>GPLGSHMSTESNDGVSETLLAWRHIDFWTSEHNPDLNATLSDPCTQNDITHAEEDLEVSFPNPVKASFKIHDGQEDLESMTGTSGLFYGFQLMTLDQVVAMTQAWRNVAKNLNKRSQQGLSHVTSTGSSSDMERLNGNKFKLPNIPDQKSIPPNAVQPVYAHPAWIPLITDNAGNHIGVDLAPGPNGKYAQIITFGRDFD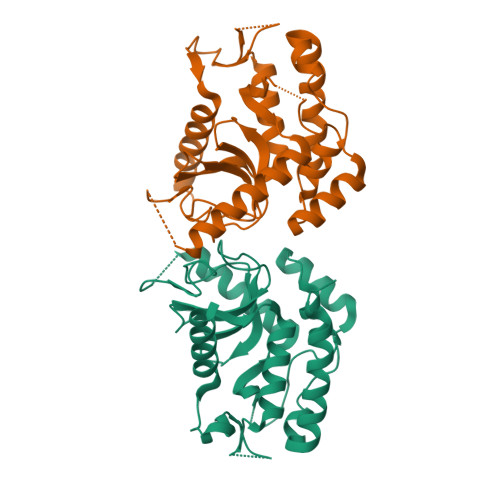TKFVIAENWGEFLLSFANDLEAGNWYLVDDNDDYFSGDGELVFRDKKSNGPIQDYFEVLKRRTWIKYQLERPHRD[2x]3-[5-(AMINOMETHYL)-4-(CARBOXYMETHYL)-1H-PYRROL-3-YL]PROPANOIC ACID | C10 H14 N2 O4 | 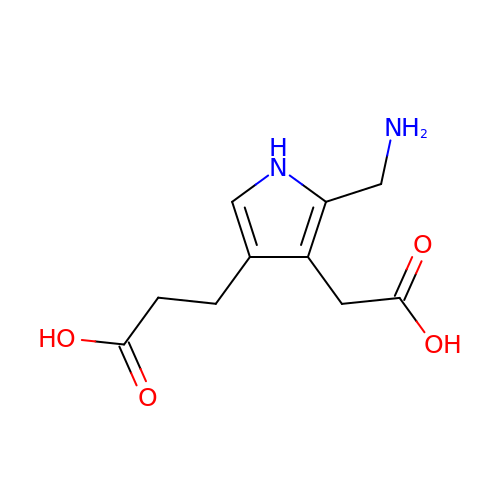QSHWIQZFGQKFMA-UHFFFAOYSA-N> MSVNYAAGLSPYADKGKCGLPEIFDPPEELERKVWELARLVWQSSSVVFHTGAGISTASGIPDFRGPHGVWTMEERGLAPKFDTTFESARPTQTHMALVQLERVGLLRFLVSQNVDGLHVRSGFPRDKLAELHGNMFVEECAKCKTQYVRDTVVGTMGLKATGRLCTVAKARGLRACRGELRDTILDWEDSLPDRDLALADEASRNADLSITLGTSLQIRPSGNLPLATKRRGGRLVIVNLQPTKHDRHADLRIHGYVDEVMTRLMKHLGLEIPAWDGPRVLERALPPLPRPPTPKLEPKEESPTRING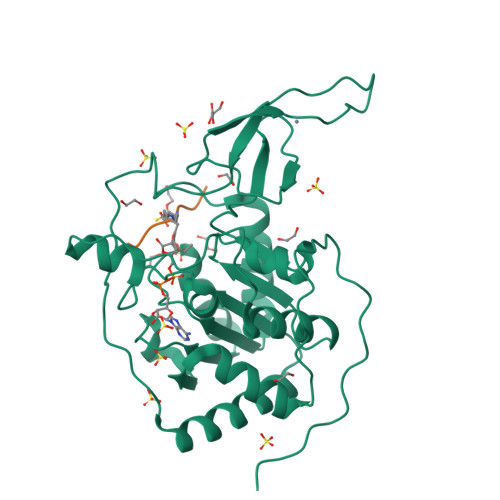SIPAGPKQEPCAQHNGSEPASPKRERPTSPAPHRPPKRVKAKAVPS;> QTARKSTGG> MSNIETVPASIEMKPNPTITVFERSPDGGRGLARDMPVRWALEEVGQPYHVRRLSFEAMKEASHLAYQPF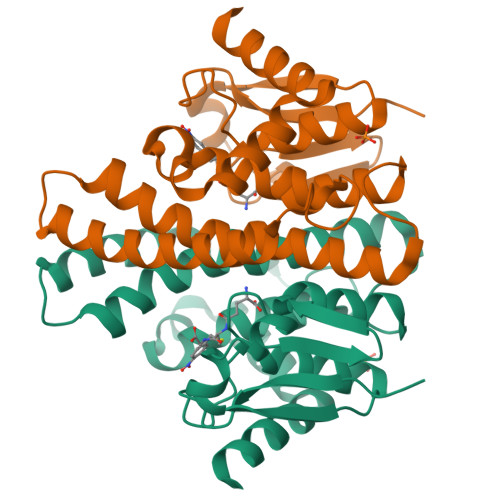GQIPSYEQGDLILFESGAIVMHIAQHHSGLLPEDQLRRARTVAWMFAALNTIEPSILNFTTVWLFERNEPWHEARLARTKEQLLKRLDELSAWLGDREWLEGSFSAADILMICVLRRLESSGILKDYGNLLAYVERGKARPAFKRAFDAQLAVFTAASKN4-oxo-N-[(1S)-1-(pyridin-3-yl)ethyl]-4-(thiophen-2-yl)butanamide 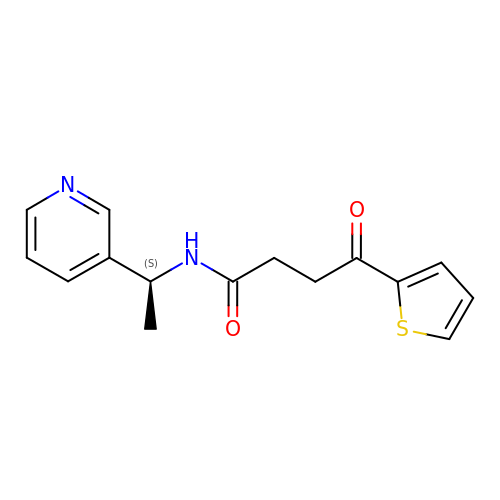| C15 H16 N2 O2 S | VFHVMIRVNCDBFW-NSHDSACASA-N>[8x]MRRTKEDSEKTRTAILLAAEELFLEKGVSHTSLEQIARAAGVTRGAVYWHFQNKAHLF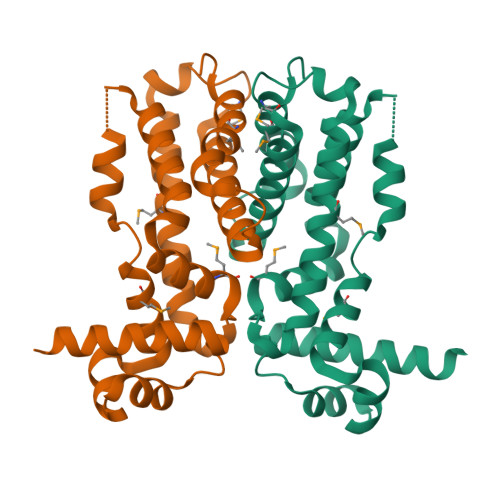NEMLNQVRLPPEQLTERLSGCDGSDPLRSLYDLCLEAVQSLLTQEKKRRILTILMQRCEFTEELREAQERNNAFVQMFIELCEQLFARDECRVRLHPGMTPRIASRALHALILGLFNDWLRDPRLFDPDTDAEHLLEPMFRGLVRDWGQASSAP>[6x]YKKAGLQRTLVLIKPDAFERSLVAEIMGRIEKKNFKIVSMKFWSKAPRNLIEQHYKEHSEQSYF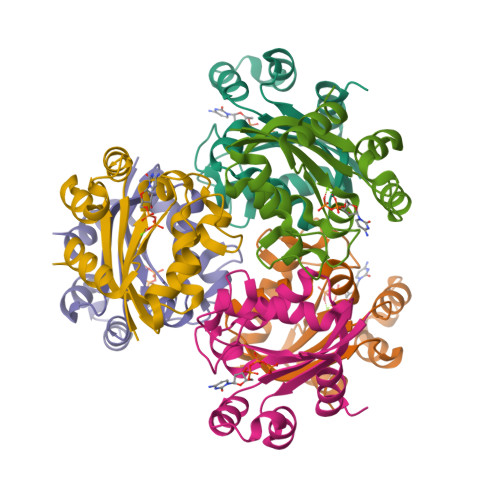NDLCDFMVSGPIISIVYEGTDAISKIRRLQGNTNPLASAPGTIRGDLANDIRENLIHASDSEDSAVDEISIWFPETKMETDN>MMKPEDVIKEQCARAKVVAELWHGFTGGAPKAALENLVVEFNKAQQGRCVRPVPQGGYRDLSTKIKAAFAAGKVPTMAQAFENNIALYLEAKALLPIESLGVKLQGVNLTFLNAVRFGGVVYGVPFNKSIQVLYYNKDLLKKHGVPVPATLEEFVAAAKKLSRAEGGPVYWFQPDASTFAYFFFNLGGSYLKDGKLVLNSKEAVEALTLLQNGVKEGWAKPITSGAINQNLGSGPYAFSVDTSAGYTYYLRAAKFDLGVATLPGRTKGQPGYGLVQGTNLVVFR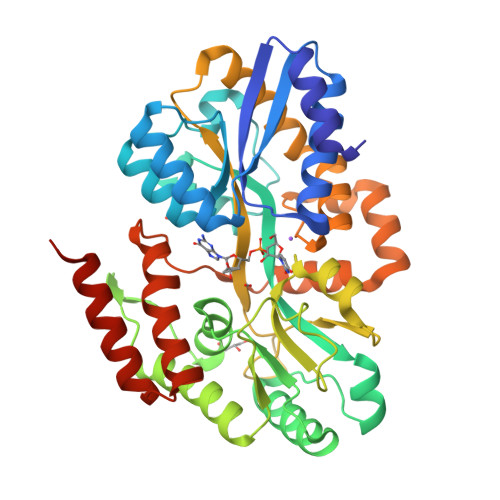QASKEEQAVAKDFLEFVLSPRAQAVFATATGYVPVTEGALKDPVYQAYAAENPDYATIVRQSRYAKFEPALAEWEQIRFDILGQAIKEAILNKADPKAALDRAQKLAEDLLSSRTRHHHHHH[2x]(3R,4R,5R)-5-(6-amino-8-bromo-9H-purin-9-yl)-3,4,5-trihydroxypentyl [(2S,3S,4S,5R)-3,4,5-trihydroxyoxolan-2-yl]methyl 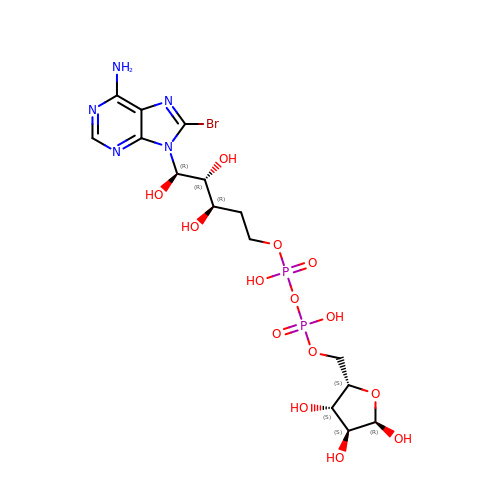dihydrogen diphosphate (non-preferred name) | C15 H24 Br N5 O14 P2 | YLKLFNYZVXTMJI-XDPXHJCRSA-N>MTHPSGEPVYADAVLNGWLTSMGLGVEYVRAEGNTVYYLDDEGREVPVLDHACGFGSLIFGHNHPEIIAHAKAALDAGTVVHAQLSRQPRANQISRILNDIMRRETGRDDRYNAIFANSGAEANEICMKHAELERQERITALFAEIDAELDTAREALTTGTATLDTASLPLVGGGAGDVDGVIADIHRHNDERRAERPLFLTLDGSFHGKLVGSIQLTQNEPWRTPFTALSSPARFLPADEPELIGKIVEDERRSVLTLSLDKDTVRVVERDFPVVAAIFVEPVRGGSGMKTVTPELAEELHRLRDTLGCPLVVDEVQTGIGRTGAFFGSALLGIRGDYYTLAKAIGGGIVKNSVALIRQDRFLPAMEVIHSSTFAKDGLSASIALKVLEMVEADGGRVYQRVRERGQRLEAMLESVRADH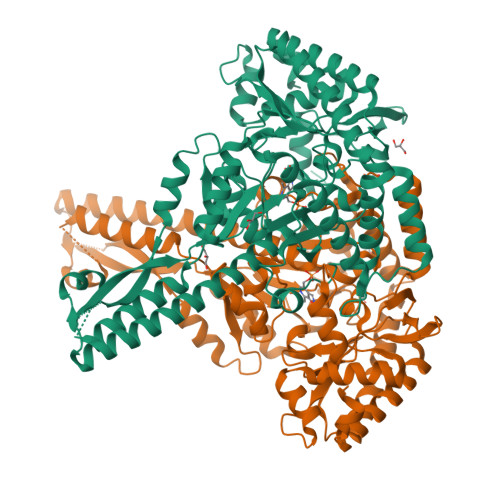SDVVSAVWGTGLMLALELRDQSNATSQAIREKAAHGFLGYVLAGFLLREHHIRVLPAGPRSGFLRFSPSLYITDEEIDRTETALRSLFTALRDQDGDRLVLS[4x]>[2x]GSRMCGNNMSTPLPAIVPAARKATAAVIFLHGLGDTGHGWAEAFAGIRSSHIKYICPHAPVRPVTLNMNVAMPSWFDIIGLSPDSQEDESGIKQAAENIKALIDQEVKNGIPSNRII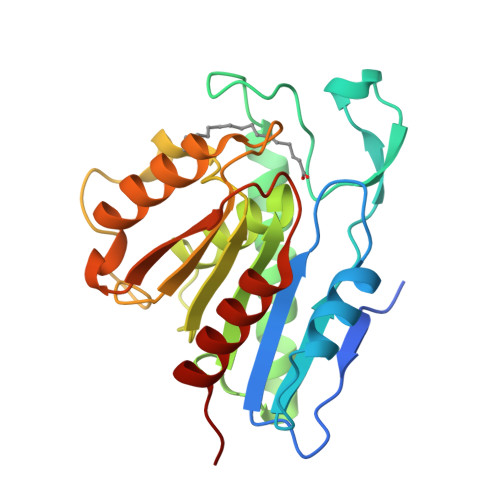LGGFAQGGALSLYTALTTQQKLAGVTALSCWLPLRASFPQGPIGGANRDISILQCHGDCDPLVPLMFGSLTVEKLKTLVNPANVTFKTYEGMMHSSCQQEMMDVKQFIDKLLPPID>[2x]MEELQDDYEDMMEENLEQEEYEDPDIPESQMEEPAAHDTEATATDYHTTSHPGTHKVYVELQELVMDEKNQELRWMEAARWVQLEENLGENGAWGRPHLSHLTFWSLLELRRVFTKGTVLLDLQETSLAGVANQLLDRFIFEDQIRPQDREELLRALLLKHSHAGELEALGGVKPAVLTRSGDPSQPLLPQHSSLETQLFCEQGDGGTEGHSPSGILEKIPPDSEATLVLVGRADFLEQPVLGFVRLQEAAELEAVELPVPIRFLFVLLGPEAPHIDYTQLGRAAATLMSERVFRIDAYMAQSRGELLHSLEGFLDCSLVLPPTDAPSEQALLSLVPVQRELLRRRYQSSPAKPDSSFYKGLDLNGGPDDPLQQTGQLFGGLVRDIRRRYPYYLSDITDAFSPQVLAAVIFIYFAALSPAITFGGLLGEKTRNQMGVSELLISTAVQGILFALLGAQPLLVVGFSGPLLVFEEAFFSFCETNGLEYIVGRVWIGFWLILLVVLVVAFEGSFLVRFISRYTQEIFSFLISLIFIYETFSKLIKIFQDHPLQKTYNYNVLMVPKPQGPLPNTALLSLVLMAGTFFFAMMLRKFKNSSYFPGKLRRVIGDFGVPISILIMVLVDFFIQDTYTQKLSVPDGFKVSNSSARGWVIHPLGLRSEFPIWMMFASALPALLVFILIFLESQITTLIVSKPERKMVKGSGFHLDLLLVVGMGGVAALFGMPWLSATTVRSVTHANALTVMGKASTPGAAAQIQEVKEQRISGLLVAVLVGLSILMEPILSRIPLAVLFGIFLYMGVTSLSGIQLFDRILLLFKPPKYHPDVPYVKRVKTWRMHLFTGIQIICLAVLWVVKSTPASLALPFVLILTVPLRRVLLPLIFRNVELQCLDADDAKATFDEEEGRDEYDEVAMPV;> MGQALGIKSCDFQAARNNEEHHTKALSSRRLFVRRGQPFTIILYFRAPVRAFLPALKKVALTAQTGEQPSKINRTQATFPISSLGDRKWWSAVV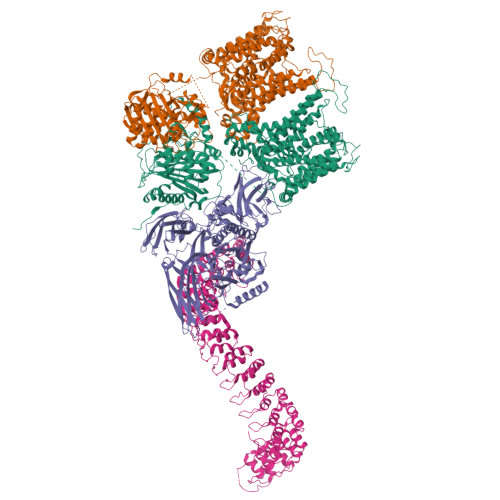EERDAQSWTISVTTPADAVIGHYSLLLQVSGRKQLLLGQFTLLFNPWNREDAVFLKNEAQRMEYLLNQNGLIYLGTADCIQAESWDFGQFEGDVIDLSLRLLSKDKQVEKWSQPVHVARVLGALLHFLKEQRVLPTPQTQATQEGALLNKRRGSVPILRQWLTGRGRPVYDGQAWVLAAVACTVLRCLGIPARVVTTFASAQGTGGRLLIDEYYNEEGLQNGEGQRGRIWIFQTSTECWMTRPALPQGYDGWQILHPSAPNGGGVLGSCDLVPVRAVKEGTLGLTPAVSDLFAAINASCVVWKCCEDGTLELTDSNTKYVGNNISTKGVGSDRCEDITQNYKYPEGSLQEKEVLERVEKEKMEREKDNGIRPPSLETASPLYLLLKAPSSLPLRGDAQISVTLVNHSEQEKAVQLAIGVQAVHYNGVLAAKLWRKKLHLTLSANLEKIITIGLFFSNFERNPPENTFLRLTAMATHSESNLSCFAQEDIAICRPHLAIKMPEKAEQYQPLTASVSLQNSLDAPMEDCVISILGRGLIHRERSYRFRSVWPENTMCAKFQFTPTHVGLQRLTVEVDCNMFQNLTNYKSVTVVAPELSA;> MPYSVGFREADAATSFLRAARSGNLDKALDHLRNGVDINTCNQNGLNGLHLASKEGHVKMVVELLHKEIILETTTKKGNTALHIAALAGQDEVVRELVNYGANVNAQSQKGFTPLYMAAQENHLEVVKFLLENGANQNVATEDGFTPLAVALQQGHENVVAHLINYGTKGKVRLPALHIAARNDDTRTAAVLLQNDPNPDVLSKTGFTPLHIAAHYENLNVAQLLLNRGASVNFTPQNGITPLHIASRRGNVIMVRLLLDRGAQIETKTKDELTPLHCAARNGHVRISEILLDHGAPIQAKTKNGLSPIHMAAQGDHLDCVRLLLQYDAEIDDITLDHLTPLHVAAHCGHHRVAKVLLDKGAKPNSRALNGFTPLHIACKKNHVRVMELLLKTGASIDAVTESGLTPLHVASFMGHLPIVKNLLQRGASPNVSNVKVETPLHMAARAGHTEVAKYLLQNKAKVNAKAKDDQTPLHCAARIGHTNMVKLLLENNANPNLATTAGHTPLHIAAREGHVETVLALLEKEASQACMTKKGFTPLHVAAKYGKVRVAELLLERDAHPNAAGKNGLTPLHVAVHHNNLDIVKLLLPRGGSPHSPAWNGYTPLHIAAKQNQVEVARSLLQYGGSANAESVQGVTPLHLAAQEGHAEMVALLLSKQANGNLGNKSGLTPLHLVAQEGHVPVADVLIKHGVMVDATTRMGYTPLHVASHYGNIKLVKFLLQHQADVNAKTKLGYSPLHQAAQQGHTDIVTLLLKNGASPNEVSSDGTTPLAIAKRLGYISVTDVLKVVTDETSFVLVSDKHRMSFPETVDEILDVSEDEGEELISFKAERRDSRDVDEEKELLDFVPKLDQVVESPAIPRIPCAMPETVVIRSEEQEQASKEYDEDSLIPSSPATETSDNISPVASPVHTGFLVSFMVDARGGSMRGSRHNGLRVVIPPRTCAAPTRITCRLVKPQKLSTPPPLAEEEGLASRIIALGPTGAQFLSPVIVEIPHFASHGRGDRELVVLRSENGSVWKEHRSRYGESYLDQILNGMDEELGSLEELEKKRVCRIITTDFPLYFVIMSRLCQDYDTIGPEGGSLKSKLVPLVQATFPENAVTKRVKLALQAQPVPDELVTKLLGNQATFSPIVTVEPRRRKFHRPIGLRIPLPPSWTDNPRDSGEGDTTSLRLLCSVIGGTDQAQWEDITGTTKLVYANECANFTTNVSARFWLSDCPRTAEAVNFATLLYKELTAVPYMAKFVIFAKMNDPREGRLRCYCMTDDKVDKTLEQHENFVEVARSRDIEVLEGMSLFAELSGNLVPVKKAAQQRSFHFQSFRENRLAMPVKVRDSSREPGGSLSFLRKAMKYEDTQHILCHLNITMPPCAKGSGAEDRRRTPTPLALRYSILSESTPGSLSGTEQAEMKMAVISEHLGLSWAELARELQFSVEDINRIRVENPNSLLEQSVALLNLWVIREGQNANMENLYTALQSIDRGEIVNMLEGSGRQSRNLKPDRRHTDRDYSLSPSQMNGYSSLQDELLSPASLGCALSSPLRADQYWNEVAVLDAIPLAATEHDTMLEMSDMQVWSAGLTPSLVTAEDSSLECSKAEDSDATGHEWKLEGALSEEPRGPELGSLELVEDDTVDSDATNGLIDLLEQEEGQRSEEKLPGSKRQDDATGAGQDSENEVSLVSGHQRGQARITHSPTVSQVTERSQDRLQDWDADGSIVSYLQDAAQGSWQEEVTQGPHSFQGTSTMTEGLEPGGSQEYEKVLVSVSEHTWTEQPEAESSQADRDRRQQGQEEQVQEAKNTFTQVVQGNEFQNIPGEQVTEEQFTDEQGNIVTKKIIRKVVRQIDLSSADAAQEHEEVTVEGPLEDPSELEVDIDYFMKHSKDHTSTPNP>[4x]MSKTFAEIAEAFLEPEAVRIAKEAVEEYGDHERKIIQIGIHFQVCCMFCDEYLSTNGSDRFVLIEGRKRGTAVSLQNELCKSYDLEPLPFLCDIFDREEKQFVEIGITRKADDSYFQSKFGKLGNSCKIFVFSYDGRLDKNCEGPMEEQKLRIFSFLATAADFLRKENMFNEIFLPDNEETIIEMKKGKTFLELRDESVPLPFQTYEQMKDYCEKFKGNPRELASKVSQMQSNIKLPIKHYEQNKFRQIRLPKGPMAPYTHKFLMEEAWMFTKISDPERSRAGEILIDFFKKGNLSAIRPKDKPLQGKYPIHYKNLWNQIKAAIADRTMVINENDHSEFLGGIGRASKKIPEISLTQDVITTEGLKQSENKLPEPRSFPRWFNAEWMWAIKDSDLTGWVPMAEYPPADNELEDYAEHLNKTMEGVLQGTNCAREMGKCILTVGALMTECRLFPGKIKVVPIYARSKERKSMQEGLPVPSEMDCLFGICVKSKSHLNKDDGMYTIITFEFSIREPNLEKHQKYTVFEAGHTTVRMKKGESVIGREVPLYLYCRTTALSKIKNDWLSKARRCFITTMDTVETICLRESAKAEENLVEKTLNEKQMWIGKKNGELIAQPLREALRVQLVQQFYFCIYNDSQLEGFCNEQKKILMALEGDKKNKSSFGFNPEGLLEKIEECLINNPMCLFMAQRLNELVIEASKRGAKFFKTD;>MEINPYLMFLNNDVTSLISTTYPYTGPPPMSHGSSTKYTLETIKRTYDYSRTSVEKTSKVFNIPRRKFCNCLEDKDELVKPTGNVDISSLLGLAEMMEKRMGEGFFKHCVMEAETEILKMHFSRLTEGRQTYDWTSERNMPA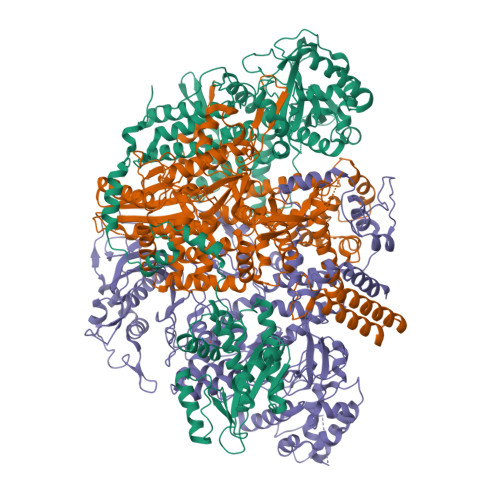ATALQLTVDAIKETEGPFKGTTMLEYCNKMIEMLDWKEIKFKKVKTVVRREKDKRSGKEIKTKVPVMGIDSIKHDEFLIRALTINTMAKDGERGKLQRRAIATPGMIVRPFSKIVETVAQKICEKLKESGLPVGGNEKKAKLKTTVTSLNARMNSDQFAVNITGDNSKWNECQQPEAYLALLAYITKDSSDLMKDLCSVAPVLFCNKFVKLGQGIRLSNKRKTKEVIIKAEKMGKYKNLMREEYKNLFEPLEKYIQKDVCFLPGGMLMGMFNMLSTVLGVSTLCYMDEELKAKGCFWTGLQSSDDFVLFAVASNWSNIHWTIRRFNAVCKLIGINMSLEKSYGSLPELFEFTSMFFDGEFVSNLAMELPAFTTAGVNEGVDFTAAMSIIKTNMINNSLSPSTALMALRICLQEFRATYRVHPWDSRVKGGRMKIINEFIKTIENKDGLLIADGGKLMNNISTLHIPEEVLKFEKMDEQYRNRVFNPKNPFTNFDKTIDIFRAHGPIRVEENEAVVSTHSFRTRANRTLLNTDMRAMMAEEKRYQMVCDMFKSVFESADINPPIGAMSIGEAIEEKLLERAKMKRDIGAIEDSEYEEIKDIIRDAKKARLESR[4x];>MSLLLTIAKEYKRLCQDAKAAQMMTVGTVSNYTTFKKWTTSRKEKNPSLRMRWAMSSKFPIIANKRMLEEAQIPKEHNNVALWEDTEDVSKRDHVLASASCINYWNFCGPCVNNSEVIKEVYKSRFGRLERRKEIMWKELRFTLVDRQRRRVDTQPVEQRLRTGEIKDLQMWTLFEDEAPLASKFILDNYGLVKEMRSKFANKPLNKEVVAHMLEKQFNPESRFLPVFGAIRPERMELIHALGGETWIQEANTAGISNVDQRKNDIRAVCRKVCLAANASIMNAKSKLVEYIKSTSMRIGETERKLEELILETDDVSPEVTLCKSALGGQLGKTLSFGPMLLKKISGSGVKVKDTVYIQGVRAVQFEYWSEQEEFYGEYKSATALFSRKERSLEWITIGGGINEDRKRLLAMCMIFCRDGDYFKDAPATITMADLSTKLGREIPYQYVMMNWIQKSEDNLEALLYSRGIVETNPGKMGSSMGIDGSKRAIKSLRAVTIQSGKIDMPESKEKIHLELSDNLEAFDSSGRIVATILDLPSDKKVTFQDVSFQHPDLAVLRDEKTAITKGYEALIKRLGTGDNDIPSLIAKKDYLSLYNLPEVKLMAPLIRPNRKGVYSRVARKLVSTQVTTGHYSLHELIKVLPFTYFAPKQGMFEGRLFFSNDSFVEPGVNNNVFSWSKADSSKIYCHGIAIRVPLVVGDEHMDTSLALLEGFSVCENDPRAPMVTRQDLIDVGFGQKVRLFVGQGSVRTFKRTASQRAASSDVNKNVKKIKMSNARENLYFQ[4x]> MWHYTSINNDTRVALDPKPNQIRTITKPNTVPQLGTDYLYTFNSQRRSHTLRLLGPFQYFNFSETDRGHPLFRLPLKYPSKAIPADELIDNLHSWMRSVHLLHVRSEDNTLRYNWMLGVYARSTNYTTPVGQLVVNAPAILNYSNPQDAFNSVFVALGIDYIDIPITNSNIFDDSSTPYNVRIWHAPTMTEVNHILALMRKSTLVSTHSSWHWNVLHTFHYRSESDMIDHFAAKILEDWRQKEKLDKGALVEADRVIQRLIPLSSSTYVQRLAAIGALYPNEFTENVLDLSRLSTALLQLSDTYYQHANDQLRRLYRRMYNDSRTLYMTQRHQELLLAQITADPNILLYPYTYIFTTIPTSMNYISNTGQGRIKHSLTVTGATEHDTVADIVLGQTGEDVITISMVEPMSIAVEDMYGYVLDTPTRDIWPADEQIEQKGDAVALYDTKTSRALGMFNNTVRIDDLLSPLLSLVYRTYIKGDTMTMTQGSLDHLTLCAAVDSDITFVGNRMIAPLPEGYIPKPMHRNNSTMKMLSLYVALKKLENFATNSYLMAPDTSIILLGAEREPAVNILRRFNRNVSNVRIIGMGDRAVEPNIRVRVPFPIDKNISADFIICDINSYEDQSFESMFSETISVVTTCASAATRALVKINHPSEYMINSVIERLSQLGGVFYHTALLKTASQNPYSYETYIYITPIAAAVRFPFYSNSAMINRYMTAVADDEMPIIPSIHTVIKGHSNTYSPGLFCGCVDVQSAPLALSQLKSYCSEATTWRVDSDDNLVNIIARIDPARIALEFRTRSNTSAYHEYQRYVPNGLGFKVRKTREFRYMHREVTFIHKLMMYALIREQISLTENMTQVVSIGGRNLADISVVPLNMKYVVIDPATRIETLTQEKKNIEVQSRPFQFDAANMDLENNSIYLFIAVIMNEPNGAATPARMQMDKIRNVATAMLTRTNCVAYISFYEAGIITRLDQSTAHKTIRVEEGRLKVANYVPVDTLVEADVTLMLRDIGITHEIIRPSTPELIDACSNYGIRLGSTGGAVLDVFNHYSPVIKLVRS;>MHSTNNNSNKRNNEEKHKQPEIDSSANNGEGTSGTRAQTVGDTATEAGVRNETKAGASTRRQTDGTGLSGTNAKIATASSARQTDVEKPADVTFTIENVDDVGIMQQKKPPTVVQSRTDVFNEQFANEALHPMTKVIFNGLDVNTEVQPLSDDFKQISDPKGYLTYSVKYEDQFTKKDKLRASEADDRIVGPTVNLFKYGAAVVNIDLNRDFFDTATGIDLTKGIPLVQDLLVPIGVTAGAEQSAEYVSGLLMVLFKVMTDNRLVIVGETTTPMSNTLSTVVNNVLRTTYHNNVGVNPALLRDFTQVNWLNRDITNMLQQAGTKYGLGLTETRLDYVRLVKTIVGHALNIDHFAASVLNINLRALMEANVTADDRIKALQAHSMISTQFHGPNQGALRPELAFDHDHIIRCLMLAAANYPRLEGIIVQINTGYVASANVIRPVSEKRYFPENLEQNQSAARLVSAVKARASEADISSIHLAIAREVSPMFNVHELKKIAESFEDPSSIVVVLEFILFALFFPTEFNRIKGDIQNVLLLFFSRWYPVEYGIFIQRGATYTINAAGEFEFSGRNEKWDQSLYLSEHFPALFSDVPLAGANTIIAIMRLFTPQGFLRTDDLAIAANFPRASRNPQTYIPYTNQRGTVTNEFASRFRTIVATLANVVNERAVQDDMQKATRSCTKQWLRHLETQFDNIAVAHTDHLSVVYATMSNFMLNFTNNFSGNHATFKPDQYVITSPEGSYKPIIERQGETVDGLTIIDTSIVWPILCQCTYPLVRQSGKGVDAVSIMEEIVYPDPSTTLSQSLSVAQVLSKLTLPDAFINMILSGGDSVVMRTYQTEADDDLDEGIRMTTYDQYLSHIRERLHITNVPDPIYITGASTPDQIAASVQATHVAVVLYQSGVINGSASTYLRENEVLVVMPDYYDVVSRFANANLQMNNNRYHESVLEIADIFDQADFIQTSDAVRQLRALMPTLSTSQIRHAIERIAQITDVDSTDYGKLTLRFLGTLTRSLKMQNAQIRRIRPDGTVLRYDDQIDIEAFRWSRYFLDELRLRRLSVGLRLITNPRIARRFDGVRIMYLTDDDPDPDFVPDVPEGYVAVQYAHRLFSSSLANKRNRVTYTHPPTGMAYPSPTGRPHVHMTINERAGMSKLVADNIIASVIKSNWVVDIHDIEYTAEVMTPSEGYTQHVDAESIMTAPKGKLFHLQFMDGLLRPEPSAFDPPASGEDMRLIYPLQPISVARSMRAIVNHNEVDRPRGAVAPSSYEMDTGTLSRNGDLLYSPVANGQVGIPKLEVDHISFSNVVSMMTANIRTGDDMAVERVNPDDVRAINIRNA[2x];>MLQQPTGGYTTLEQFAFTIRNDGTNATPTQFLQLLSYEATENELVKKTIPTPETHLPSARNVPGNVYIEDAITQALFGISAQNVNAHGYFSRLSALALPNTSARLGLDGVIYNSETINIPFYDPAAVANFAATYAKLGNASTPRYRADMIDIYAHVGLELAGTDAERAAGVMPVKRAKFDSWEGSLISLSRDVVNWKILAFLIDLCSLEGEALRAFKTRNRDVFRMMLFIMSTAVAANVVNRKVTKRVDRVLEYIGVNSMRTAGRTATITYDLSRHEFAAKFLQLTFTRWNAASAMIRSMPDMHTPRTSITPAGENALVRHNRYMTENFKGLSPIALAQKKHEMMLHTHE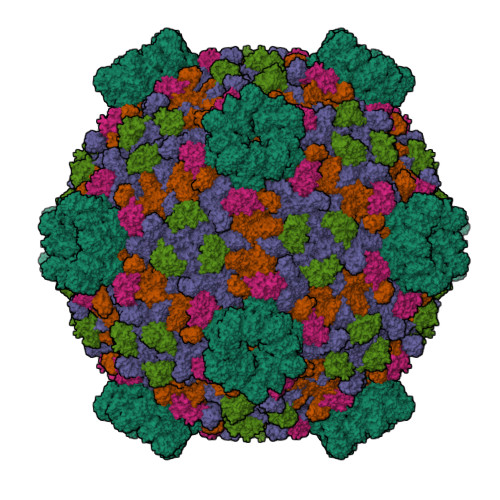IHSMDIDGSIKNMVERETVNKMNEIDAMNTAPWTEEFAEVEPTTVYERHQIGTDPEQTQLISQDAAVIVHQASSDVDENEYGNSVSELTIDTQSDSVL[2x]>GTLTGERPPVFWLQGQGCTGCSVTLLNSVHPSIADVLLKVISLEFHPTVMAWEGEHAIEHMRKVAEKFKGKFFLVIEGSVPVEADGKYCIIGEANHHEISMVDALKEFGPNAAAVLAVGTCAAYGGIPAAEGSETGATAVSKFLGDNGIKTPVVNIPGCPPHPDWIVGTVVLALDAIKKNGLEGGLAEVVKVLDSDGRPTPFFGRNIHENCPYLDKYDEGVMSATFTDKVGCRYDLGCKGPMTMADCFERKWNGGVNWCVQNAVCIGCVEPDFPDGKSPFYQA[4x];>[4x]GATGRTTIAIDPVTRIEGHLKAEVVVENGKVVDARLSGGMYRGFETILRGRDPRDASQIVQRICGVCPTAHSTASVLALDEAFGAKVPNNGRITRNLIFGANYLQSHILHFYHLSAQDFVQGPDTAPFVPRFPKSDLRLSKELNKAGVDQYIEALEVRRICHEMVALFGGRMPHVQGQVVGGATEIPTKEKLVEYAARFKKVRDFVEQKYVPVVYTIGSKYKDMFKVGQGFKAALCVGAFPLDNSGKKHLFMPGVYAKGKDMPFDPSKIKEYVKYSWFAEETTGLNYKEGKTIPAPDKAGAYSFVKAPRYDGLSLEVGPLARMWVNNPELSPVGKKLLKDLFGISAKKFRDLGEEAAFSLMGRHVARAEETYYMLGAIEGWLKEIKAGEDTVVMPAVPASAEGTGFTEAPRGSLLHYVKVKDSKIDNYQIVSASLWNCNPRDDMGQRGAVEEALIGIPVDDI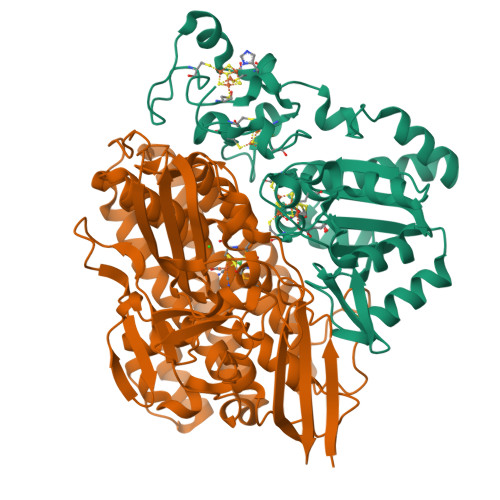QNPVNVARLIRAFDPULACAVH>MQRWPKYGGTDVNTRTVHDLLNTINTMSARIKTLERYEHALREIHKVVVILKPSANTHSFEPDALPALIMQFLSDFAGRDINTLTHNINYKYDYNYPPAPVPAMQPPPPPPQPPAPPQPPYYNNYPYYPPYPFSTPPPTQPPESNVAGVGGSQSLNQITLTNEEESELAALFKNMQTNMTWELVQNFVEVLIRIVRVHVVNNVTMINVISSITSVRTLIDYNFTEFIRCVYQKTNIRFAIDQYLCTNIVTFIDFFTRVFYLVMRTNFQFTTFDQLTQYSNELYTRIQTSILQSAAPLSPPTVETVNSDIVISNLQEQLKRERALMQQISEQHRIANERVETLQSQYDELDLKYKEIFEDKSEFAQQKSENVRKIKQLERSNKELNDTVQKLRDENAERLSEIQLQKGDLDEYKNMNRQLNEDIYKLKRRIESTFDKDYVETLNDKIESLEKQLDDKQNLNRELRSSISKIDETTQRYKLDAKDIMELKQSVSIKDQEIAMKNAQYLELSAIYQQTVNELTATKNELSQVATTNQSLFAENEESKVLLEGTLAFIDSFYQIIMQIEKPDYVPISKPQLTAQESIYQTDYIKDWLQKLRSKLSNADVANLQSVSELSDLKSQIISIVPRNIVNRILKENYKVKVENVNAELLESVAVTSAVSALVQQYERSEKQNVKLRQEFEIKLNDLQRLL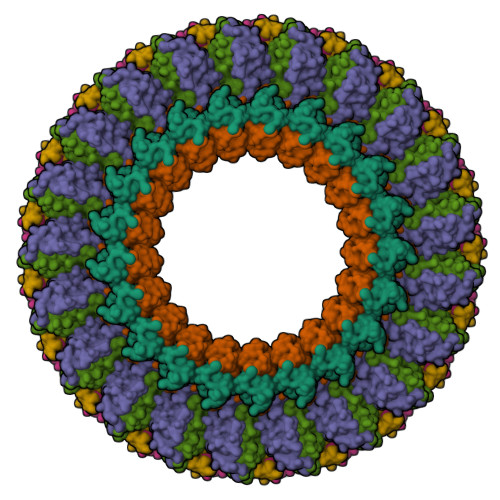EQNQTDFESISEFISRDPAFNRNLNDERFQNLRQQYDEMSSKYSALETTKIKEMESIADQAVKSEMSKLNTQLDELNSLFVKYNRKAQDIFEWKTSMLKRYETLARTTAASVQPNVE[2x];>[2x]MIASINDTDMDTDDNMSQARRNRRNRPPARPSAQTQMAAVDMLQTINTAASQTAASLLINDITPNKTESLKILSTQSVGARSLLEPMQANASTIKLNRIETVNVLDFLGSVYDNTIQVIVTE;>MSAIALYLEINKLRLKIDEPMQLAIWPQLFPLLCDEHQSVQLNTDVLINFMMHVARKSQNTILNNNAAIASQYAAGNADVVAAPASAQPTPRPVINLFARANAAAPAQPSEELINMRRYRNAARKLIHHYSLNSTSSTEYKISDVVMTMIFLLRSEKYHSLFKLLETTFDDYTCRPQMTQVQTDTLLDAVRSLLEMPSTTIDLTTVDIMRSSFARCFNSPIMRYAKIVLLQNVALQRDKRTTLEELLIERGEKIQMLQPQQYINSGTEIPFCDDAEFLNRLLKHIDPYPLSRMYYNAANTMFYTTMENYAVSNCKFNIEDYNNIFKVMENIRKHSNKNSNDQDELNIYLGVQSSNAKRKKY[2x]> PSFDCGKPQVEPKKCPGRVVGGCVAHPHSWPWQVSLRTRFGMHFCGGTLISPEWVLTAAHCLEKSPRPSS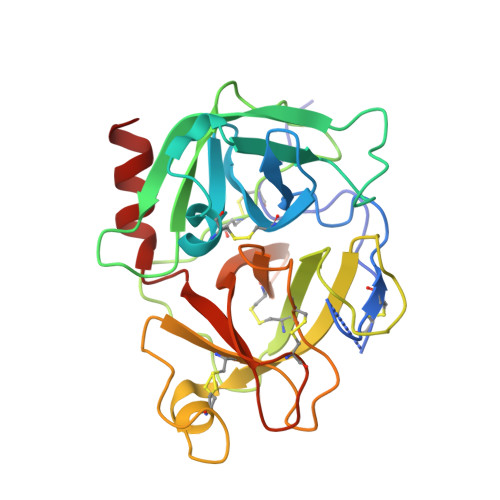YKVILGAHQEVNLEPHVQEIEVSRLFLEPTRKDIALLKLSSPAVITDKVIPACLPSPNYVVADRTECFITGWGETQGTFGAGLLKEAQLPVIENKVCNRYEFLNGRVQSTELCAGHLAGGTDSCQGDSGGPLVCFEKDKYILQGVTSWGLGCARPNKPGVYVRVSRFVTWIEGVMRNN>GAMDPEFMSTPLPAIVPAARKATAAVIFLHGLGDTGHGWAEAFAGIRSSHIKYICPHAPVRPVTLNMNVAMPSWFDIIGLSPDSQEDESGIKQAAENIKALIDQEVKNGIPSNRIILGGFSQGGALSLYTALTTQQKLAGVTALSCWLPLRASFPQGPIGGANRDISILQCHGDCDPLVPLMFGSLTVEKLKTLVNPANVTFKTYE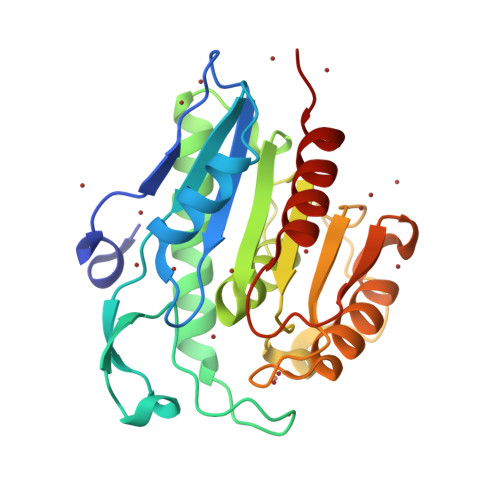GMMHSSCQQEMMDVKQFIDKLLPPID[2x]> ENLTPQHMASMALTGTDRVKRGMAEMQKGGVIMDVVNAEQAKIAEAAGAVAVMALERVPADIRAAGGVAR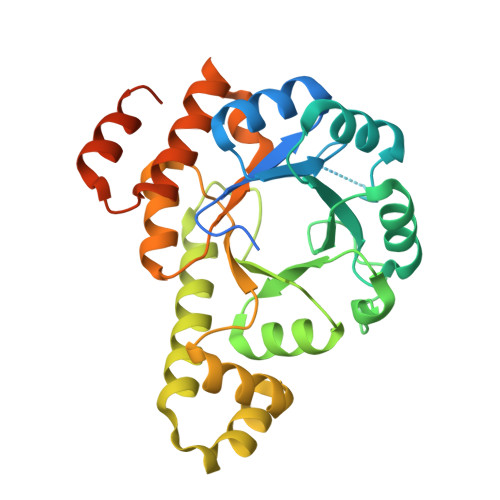MADPTVIEEVMNAVSIPVMAXVRIGHYVEARVLEALGVDYIDESEVLTPADEEFHIDKRQFTVPFVCGCRDLGEAARRIAEGASMLRTKGEPGTGNIVEAVRHMRKVNAQIRKVVNMSEDELVAEAKQLGAPVEVLREIKRLGRLPVVNFAAGGVTTPADAALMMHLGADGVFVGSGIFKSENPEKYARAIVEATTHYEDYELIAHLSKGLGGAMRGIDIATLLPEHRMQERGW>SKTKAFTIPVLKISEMTNSRFPVPVDQMYTSRSEGIVVQPQNGRATIDGELLGTTLVSPVSVCNFKGNLQAEVPGQHQLYQLQLTNLDGSPIDPTDDTPGPLGCPDFTGLLYGVASQRGPGDATRAHEARIDTGSDTFAPKIGQVRFYSTSSDFETNQPTHFTPIGIYIEGNSSDFNQWQLPRYGGHLANNNHLAPAVSPLFPGEQILFFRSFIPGASGHTNGEMDCLLPQEFVQHFYQEAATARSEVALLRFVNPDTGRALFESKLHKQGFMTIASSGDHPIIMPTNGYFRFEAWVNQFYSLAPVGTGSG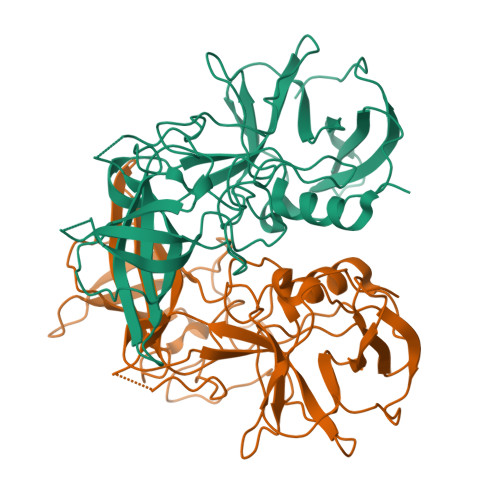RRRIQ[2x]Src homology 3 (SH3)-domain growth factor receptor-bound 2-like (endophilin) interacting protein 1 (SGIP1) and its splicing variant, SGIP1α, are brain-specific homologs of FCHo1/FCHo2. The μHDs of SGIP1 and SGIP1α, which are identical to each other, are highly homologous to those of FCHo1/FCHo2. The μHD of SGIP1/SGIP1α also binds to the DPF motif-rich region of Eps1519. Thus, the SGIP1/FCHo1/FCHo2 μHD is a domain designed for recognizing the locally ordered structure formed by the two consecutive DPF motifs.

To gain further insights into the mechanism of DPF-motif recognition by the μHD, we solved the crystal structures of the SGIP1 μHD in two different space groups. The two structures are similar to each other, and the minor differences in the secondary structure composition are probably due to crystal packing effects. The structure of the SGIP1 μHD adopts a topology similar to those of the previously determined μHD structures. However, the SGIP1 μHD possesses unique structural features that distinguish it from the other known μHD structures. Among these distinctive features, the most prominent one is the presence of the SGIP1/FCHo1/FCHo2-specific insertion of a relatively long α-helix (α2) between β6 and β7. Due to this insertion, the loop between α2 and β7 and the N-terminal part of β7 also adopt conformations strikingly different from those in other μHDs. Since these regions contain critical Eps15 interacting residues (see below), these unique structural features of the SGIP1 μHD are functionally relevant.

> GPLGSLTMGAQDTLPVAAAFTETVNAYFKGADPSKCIVKITGEMVLSFPAGITRHFANNPSPAALTFRVINFSRLEHVLPNPQLLCCDNTQNDANTKEFWVNMPNLMTHLKKVSEQKPQATYYNVDMLKYQVSAQGIQSTPLNLAVNWRCEPSSTDLRIDYKYNTDAMTTAVALNNVQFLVPIDGGVTKLQAVLPPAVWNAEQQRILWKIPDISQKSENGGVGSLLARFQLSEGPSKPSPLVVQFTSEGSTLSGCDIELVGAGYRFSLIKKRFAAGKYLADN>[4x]MEHHHHHHATNLRGVMAALLTPFDQQQALDKASLRRLVQFNIQQGIDGLYVGGSTGEAFVQSLSEREQVLEIVAEEAKGKIKLIAHVGCVSTAESQQLAASAKRYGFDAVSAVTPFY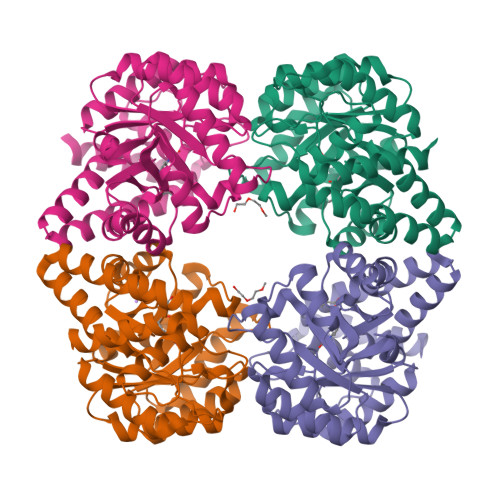YPFSFEEHCDHYRAIIDSADGLPMVVFNIPALSGVKLTLDQINTLVTLPGVGALKQTSGDLYQMEQIRREHPDLVLYNGYDNIFASGLLAGADGGIGSTYNIMGWRYQGIVKALKEGDIQTAQKLQTECNKVIDLLIKTGVFRGLKTVLHYMDVVSVPLCRKPFGPVDEKYLPELKALAQQLMQERG Terminal uridylyl transferase (TUTase) is one type of enzyme that modifies RNA molecules by facilitating the post-transcriptional addition of uridyl ribonucleotides to their 3′ ends. Recent researches have reported that Drosophila TUTase, Tailor, exhibits an intrinsic preference for RNA substrates ending in 3′G, distinguishing it from any other known TUTases. Through this unique feature, Tailor plays a crucial role as the repressor in the biogenesis pathway of splicing-derived mirtron pre-miRNAs. The structure of Tailor contains two canonical globular domains separated by a large catalytic groove, which serves to accommodate the 3′ ends of the target RNAs for the post-transcriptional addition of uridyl ribonucleotides.

In this research, we determined the high-resolution crystal structures of Drosophila Tailor-C, and its complexes with UTP and three short RNA stretches (5′-AGU-3′, 5′-AGUU-3′ and 5′-UUUU-3′) using X-ray crystallography. In all these structures, RNA stretches exhibit a very similar binding mode for Tailor, lying along the canonical catalytic groove formed between the CAT and CD of Tailor with the terminal 3′Us anchored into the pocket at the bottom of the groove which is usually occupied by UTP or its analogue in previously reported structures. This is further confirmed by our structure of Tailor-UTP in which UTP can be perfectly superimposed with the terminal 3′Us in Tailor-AGU and Tailor-AGUU and maintains conserved interactions with surrounding residues. Three conserved catalytic aspartic acid residues (Asp278, Asp280 and Asp 343) sit closely with their side chains all pointing outward from the other side towards the groove.

> HMQHITVRLPKKARAMIVGEITNVFKDKYPIADKLKVIPEYDVIEQDLCKLLSPGFPKQPLRVYKFGSRITGIGNRSSDLDLFVDIGNTFHTFEHRASNATVAKLRAMRKFFCDSEDWRLINFIEQARVPIIKTCHLPTGIECAICLNSMGFCNTNLLKYIFESQPLTQYMCIYVKNWLERCKLTEQISTYSITLMVIYFLQLQALLPPIAMLQIEDAANQAVLVGPWVVNFAQKSFSELGLQQLKATVPVIKGFLRNFFAYFAKFDYEHFLVCPYIGQANVEIAKIERMLHARYSAYVSDNPECSIQLKKPMVVQDPIQLNHNVTKAVTKYGLQTFVDYCQQTAELLEEPSTNWRQRYAF> AETVSFSWNKFVPKQPNMILQGDAIVTSSGKLQLNKVDENGTPKPSSLGRALYSTPIHIWDKETGSVASFAASF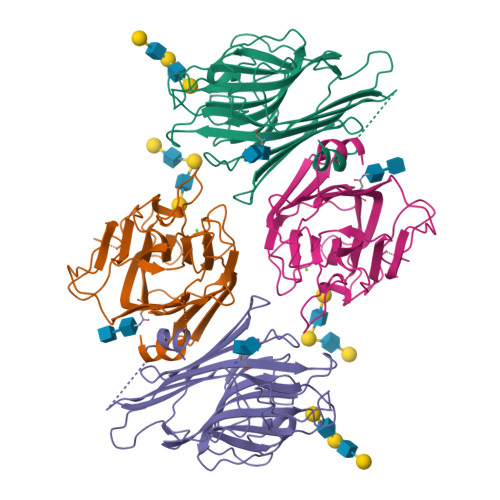NFTFYAPDTKRLADGLAFFLAPIDTKPQTHAGYLGLFNENESGDQVVAVEFDTFRNSWDPPNPHIGINVNSIRSIKTTSWDLANNKVAKVLITYDASTSLLVASLVYPSQRTSNILSDVVDLKTSLPEWVRIGFSAATGLDIPGESHDVLSWSFASNLPHASSNIDPLDLTSFVLHEAI>MTATEELTFESTSRFAEVDVDGPLKLHYHEAGVGNDQTVVLLHGGGPGAASWTNFSRNIAVLARHFHVLAVDQPGYGHSDKRAEHGQFNRYAAMALKGLFDQLGLGRVPLVGNSLGGGTAVRFALDYPARAGRLVLMGPGGLSINLFAPDPTEGVKRLSKFSVAPTRENLEAFLRVMVYDKNLITPELVDQRFALASTPESLTATRAMGKSFAGADFEAGMMWREVYRLRQPVLLIWGREDRVNPLDGALVALKTIPRAQLHVFGQCGHWVQVEKFDEFNKLTIEFLGGGRK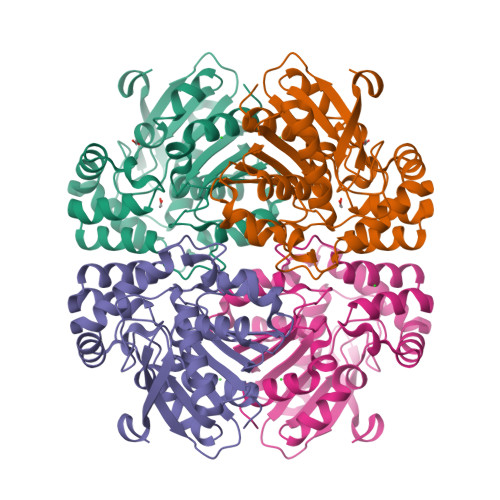LHHHHHH[2x]>[6x]MTGEDFKIKSGLAQMLKGGVIMDVVTPEQAKIAEKSGACAVMALESIPADMRKSGKVCRMSDPKMIK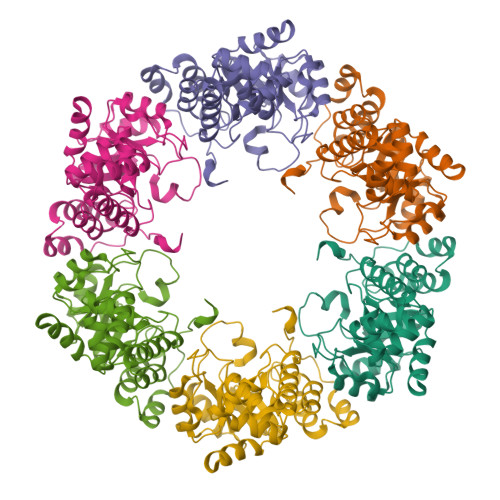DIMNSVSIPVMAKVRIGHFVEAQIIEALEVDYIDESEVLTPADWTHHIEKDKFKVPFVCGAKDLGEALRRINEGAAMIRTKGEAGTGDVSEAVKHIRRITEEIKACQQLKSEDDIAKVAEEMRVPVSLLKDVLEKGKLPVVNFAAGGVATPADAALLMQLGCDGVFVGSGIFKSSNPVRLATAVVEATTHFDNPSKLLEVSSDLGELMGGVSIESISHASNGVRLSEIGW> MRDNSDTVKMKRGINIGNALESPKDFPWDVKMSNKFFDDIKDAGFDTVRIPVRFSDYTSDSDNFKIDEDFFKKIDKYVDYALDKDLIVVLDLHHFEEIMKEPRVHKEKFLKIWQQIANRYQKYDKKLVFELLNEPKENLYS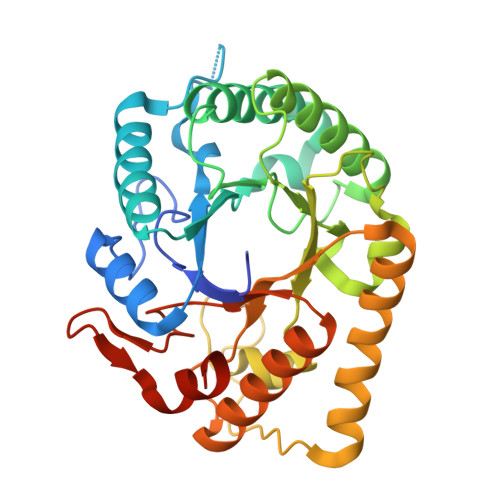QLLNEYIEEAIKIIRKTNPKRTIIVGPYNFYQIDYLNELNIPKDSNIVVSFHYYEPNDFAFQGNIYHKGFEHLSNITWEGTNEQMDYLKKRFDTVENWANKNNVKIFLGEFGVTKEAPETSRRAWVKAVREEAEKRNFSWAYWELASGFGIYNQIEGTWDRDILSALIEKRLEHHHHHH> MNGVYDVGGTDGLGPINRPADEPVFRAEWEKVAFAMFPATFRAGFMGLDEFRFGIEQMNPAEYLESPYYWHWIRTYIHHGVRTGKIDLE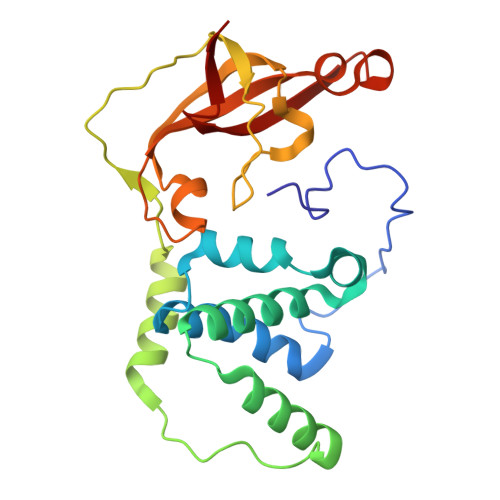ELERRTQYYRENPDAPLPEHEQKPELIEFVNQAVYGGLPASREVDRPPKFKEGDVVRFSTASPKGHARRARYVRGKTGTVVKHHGAYIYPDTAGNGLGECPEHLYTVRFTAQELWGPEGDPNSSVYYDCWEPYIELV> IVGGYECKAYSQAHQVSLNSGYHFCGGSLVNENWVVSAAHCYKSRVEVRLGEHNIKVTEGSEQFISSSRVIRHPNYSSYNIDNDIMLIKLSKPATLNTYVQPVALPTSCAPAGTMCTVSGWGNTMSSTADSDKLQCLN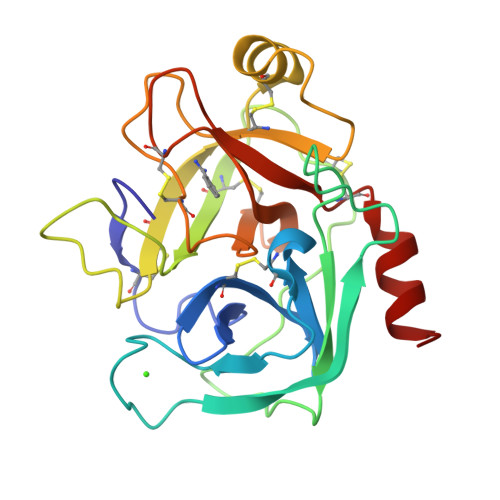IPILSYSDCNDSYPGMITNAMFCAGYLEGGKDSCQGDSGGPVVCNGELQGVVSWGYGCAEPGNPGVYAKVCIFSDWLTSTMASY> IPIFLSVLQSIE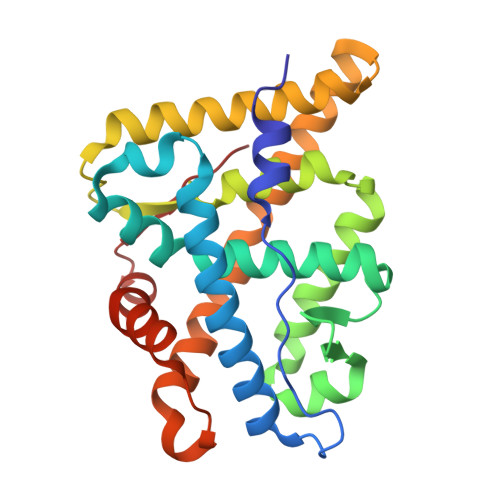PEVVYAGYDNTQPDTSASLLTSLNELGERQLVRVVKWAKALPGFRNLHVDDQMTLIQYSWMGVMVFAMGWRSYKNVNSRMLYFAPDLVFNEQRMQKSTMYNLCVRMRHLSQEFVWLQVTQEEFLCMKALLLFSIIPVEGLKNQKYFDELRMNYIKELDRVISFQGKNPTSSSQRFYQLTKLLDSLQPIVRKLHQFTFDLFVQSQSLSVEFPEMMSEIISAQVPKILAGMVKPLLFH alpha-L-idopyranuronic acid | C6 H10 O7 | 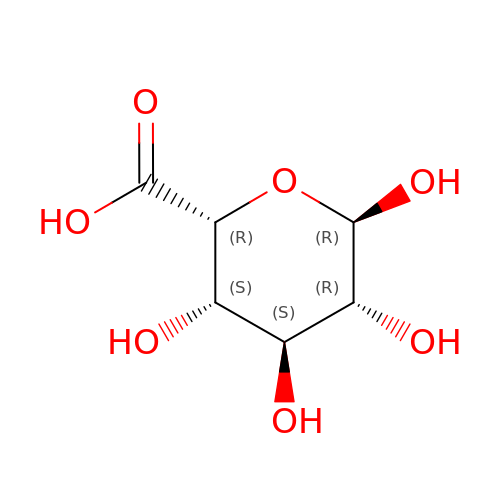AEMOLEFTQBMNLQ-VCSGLWQLSA-N2-{[(3R,4S)-3-fluoro-1-{[4-(trifluoromethoxy)phenyl]acetyl}piperidin-4-yl]oxy}-5-(1-methyl-1H-imidazol-4-yl)pyridine-3-carboxamide | C24 H23 F4 N5 O4 | 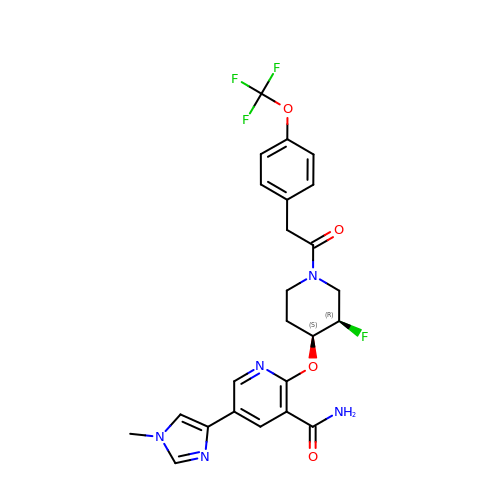XJIIVPVOGYFVME-QUCCMNQESA-N>GMSGQKPVKPSADGLLASARAIKSKGPAPVHLWNPPFNGDIDMRIARDGTWFYQGTPINRPAMVRLFSSILKREEDRFYLVTPVEKVGIRVDDAPFVAVDVEVAGQGRKQVLTFTTHVGDSAVAGEGNPIRMAQDPATGEPAPYVHVRAGLEALIDRKSFYRLMDLGEIEDGWFGLWSSGSFFPLMTVEELERG[2x]

To extend the structural coverage of proteins with uncharacterized biological function, we targeted Pfam protein family Pfam06938 (DUF1285), for which we determined the structures of two representative members. The first structural representatives of the DUF1285 family revealed a novel fold consisting of repeated motifs. The structures revealed a conserved core with domain duplication and a superficial similarity of the C-terminal domain to pleckstrin homology-like folds. The conservation of the domain interface indicates a potential binding site that is likely to involve a nucleotide-based ligand, with genome-context and gene-fusion analyses additionally supporting a role for this family in signal transduction, possibly during oxidative stress.

The SPO0140 gene of Silicibacter pomeroyi DSS-­3, a marine α-proteobacterium, encodes a protein with a molecular weight of 21.2 kDa (residues 1–193) and a calculated iso­electric point of 5.7. The crystal structure of SPO0140 was determined to 2.5 Å resolution using the MAD method. The final model included two protomers (residues 10–192 for chain A, residues 10–193 for chain B), one glycerol molecule and 186 water molecules in the asymmetric unit. SPO0140 is an α/β protein comprising two domains. The N-­terminal domain (residues 10–93) consists of a β-meander–α-­helix–β-meander core (residues 24–92), with the two β-meanders hydrogen bonding along the first and sixth strands to form a twisted mixed six-stranded β-sheet. Two N-terminal helices (H1 and H2) pack against the sheet and complete this domain. SPO0140 crystallized with two monomers (A and B) in the asymmetric unit. The largest packing interface buries ∼810 Å2 of solvent-accessible surface per monomer and involves mainly helix H1, strand β1 and the H3–β4 loop from the N-terminal domain and helix H4 and strands β14–β15 from the C-terminal domain. However, packing analysis using PISA suggests that this would not be a stable dimerization interface. The results of analytical size-exclusion chromatography (anSEC) support the assignment of a monomer as the quaternary state in solution for SPO0140.>[2x]GANTTETPVKDVELDGRWDDPIRSAATNCPITVFTD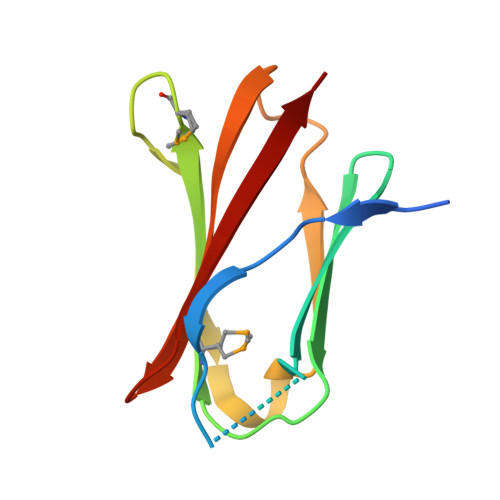GYLLTLKNASPDRDMTIRITDMAKGGVVYENDIPEVQSAYITISIANFPAEEYKLEITGTPSGHLTGYFTKE Resminostat 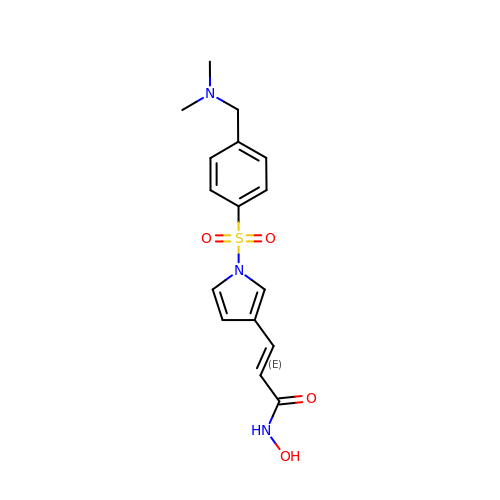| C16 H19 N3 O4 S | FECGNJPYVFEKOD-VMPITWQZSA-N Phylogenetically diverse bacteria can carry out chloramphenicol reduction, but only a single enzyme has been described that efficiently catalyzes this reaction, the NfsB nitroreductase from Haemophilus influenzae strain KW20. We found that expression of H. influenzae and Neisseria spp. nfsB genes, but not Pasteurella multocida nfsB, allows Escherichia coli to resist chloramphenicol by nitroreduction. Mass spectrometric analysis confirmed that purified H. influenzae and N. meningitides NfsB enzymes reduce chloramphenicol to amino-chloramphenicol, while kinetics analyses supported the hypothesis that chloramphenicol reduction is a secondary activity. Previous kinetic studies of nitroreductase catalysis revealed that reactions progress by a double-displacement (ping-pong) mechanism that appears to lack the gating steps necessary to impose specificity, explaining the substrate promiscuity of these enzymes.

Previous work has demonstrated that the NfsB enzyme from H. influenzae strain Rd KW20 (Hi KW20) has the ability to reduce chloramphenicol to amino-chloramphenicol in vitro. We previously demonstrated that expression of the nfsB housekeeping gene from H. influenzae KW20 (Hi KW20) is sufficient to confer clinically relevant levels of chloramphenicol resistance in Es. coli. To understand better how variation in the substrate-binding site mediates activity, we solved the crystal structures of the NfsB homologs from Hi KW20, Hi Int1, Hi 86-028NP, and Nm Z2491. We compared the activity of each NfsB homolog against Hi KW20 NfsB because it was the only previously characterized chloramphenicol reductase. Cell-free supernatants from the empty vector control and Es. coli strain expressing the Pm 70 nfsB gene reactions showed negligible derivatization by the Bratton-Marshall reagent, while supernatants from the Es. coli strains expressing H. influenzae or Neisseria nfsB genes showed robust signal, with the strain expressing the Hi KW20 nfsB showing the highest apparent reduction rate. The relative increase in resistance conferred by H. influenzae or Neisseria nfsB expression ranged from approximately a 16-fold increase (Hi KW20 and Hi 86-028NP) down to an ∼2-fold increase (Hi Int1 and Hi 12). The divergence in chloramphenicol resistance and in vitro activity likely reflect the vagaries of heterologous expression in Es. coli and suggest the presence of important subtleties that still need to be accounted for when estimating mobilization risks of cryptic and proto-resistance genes. This is especially evident with the NfsB enzymes from Hi KW20 and Hi Int1. Intuitively, the Ser68-Met74 pair found in Hi 12 NfsB would provide more of the flexibility needed to properly locate and orient Trp71 to make space for the ribose of NADP than the Pro68-Ile74 pair in other H. influenzae NfsB homologs (Pro68-Ala74 in Nm Z2491 NfsB).

>[2x]SNAMTQLTREQVLELFHQRSSTRYYDPTKKISDEDFECILECGRLSPSSVGSEPWKFLVIQNKTLREKMKPFSWGMINQLDNCSHLVVILAKKNARYDSPFFVDVMARKGLNAEQQQAALTKYKALQEEDMKLLENDRTLFDWCSKQTYIALANMLTGASALGIDSCPIEGFHYDKMNECLAEEGLFDPQEYAVSVAATFGYRSRDIAKKSRKGLDEVVKWVG> MDEFEMIKRNTSEIISEEELREVLKKDEKSAGIGFEPSGKIHLGHYLQIKKMIDLQNAGFDIIIELADLHAYLNQKGELDEIR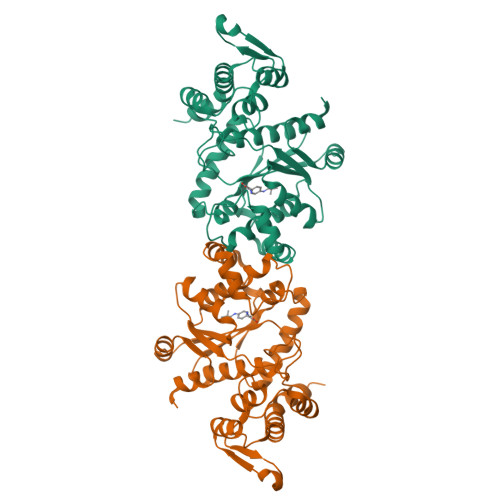KIGDYNKKVFEAMGLKAKYVYGSEFQLDKDYTLNVYRLALKTTLKRARRSMELIAREDENPKVAEVIYPIMQVNGCHYLGVDVAVGGMEQRKIHMLARELLPKKVVCIHNPVLTGLDGEGKMSSSKGNFIAVDDSPEEIRAKIKKAYCPAGVVEGNPIMEIAKYFLEYPLTIKRPEKFGGDLTVNSYEELESLFKNKELHPMDLKNAVAEELIKILEPIRKRLLEHHHHHH>MKTIFSGIQPSGVITIGNYIGALRQFVELQHEYNCYFCIVDQHAITVWQDPHELRQNIRRLAALYLAVGIDPTQATLFIQSEVPAHAQAAWMLQCIVYIGELERMTQFKEKSAGKEAVSAGLLTYPPLMAADILLYNTDIVPVGEDQKQHIELTRDLAERFNKRYGELFTIPEARIPKVGARIMSLVDPTKKMSKSDPNPKAYITLLDDAKTIEKKIKSAVTDSEGTIRYDKEAKPGISNLLNIYSTLSGQSIEELERQYEGKGYGVFKADLAQVVIETLRPIQERYHHWMESEELDRVLDEGAEKANRVASEMVRKMEQA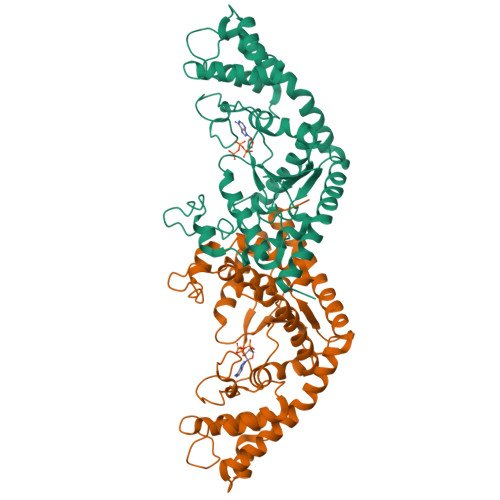MGLGRRR[6x]>[4x]MGSSHHHHHHSSENLYFQGHIETLPDSFTFYDGTKVQRLSDWPKRAQELKDLYQFYMYGYKPDTSVEDVTYSVNGNTLTITVKVGDKQASFNATVRLPQANSGYQPPYPVIISLGYLAGFNWQTWQFIDYSTNAVNRGYAVISFMPNDVARDDSSYTGAFYTLYPHSNKVENDTGVLMAWAWGASKILDALEKGAIPEIDAKKAIVTGFSRYGKAALVAGAFDERFAVVNPHASGQGGAASFRYSFAGKQYSWGVAGNAEAFSNLQGNTEGHWFNAVFREFKDPRQLPFDQHELIALCAPRTVLITGGYSDWGTNPEGTWVSFVGARKVYEFLGVADRIGFALRDGSHAITEEDVNNLLDFCDWQLRGIQPTKDFSTSRFAIDPAWDTISVPTLYRNAD

The hyperthermophilic bacterium Caldicellulosiruptor kristjansonii encodes an unusual enzyme, CkXyn10C-GE15A, which incorporates two catalytic domains, a xylanase and a glucuronoyl esterase, and five carbohydrate-binding modules (CBMs) from families 9 and 22. C. kristjansonii has been shown to grow on a variety of polysaccharides, including cellulose, xylan, starch, and pectin, with an optimal growth temperature of 78 °C. From the N-terminus, CkXyn10C-GE15A consists of two CBM22 domains (CBM22.1 and CBM22.2), a GH10 endo-xylanase (Xyn10C), three CBM9 domains (CBM9.1, CBM9.2, and CBM9.3), a GE from CE15 (GE15A), a cadherin domain, and two surface layer homology (SLH) domains believed to anchor the protein to the Gram-positive cell wall. Collectively, the results show that all five CBMs have their own distinct binding preferences and appear to complement each other and the catalytic domains in targeting complex cell wall polysaccharides. We have determined the structures of the third CBM9 domain (CBM9.3) and the glucuronoyl esterase (GE15A) by X-ray crystallography.

In addition to determining the structure of CBM9.3, we were also able through renewed efforts to crystallize and determine the structure of the previously biochemically characterized GE15 domain of CkXyn10C-GE15A.15 Residue numbers in this section reflect the numbering as in the PDB file, where Glu22 corresponds to Glu1340 in the full-length protein sequence. We were also able to determine the 3D structure of the GE domain, which represents the first structure of a GE from a hyperthermophilic organism. As expected from previously determined structures of CE15 enzymes, the overall structure is an α/β-hydrolase fold with the active site located in a shallow pocket, and as in other studied bacterial GEs, there are no disulfide bonds. Within the active site, the catalytic serine-histidine-glutamate/aspartate triad is conserved and easily identifiable in CkGE15A and is comprised of Ser210, His348, and Asp311. Compared to previously studied GEs, one of the major differences in CkGE15A is that it lacks two inserts previously found in bacterial enzymes (Reg1 and Reg3) and has a rather different structure of the aromatic-rich Reg2, implicated in the interaction with the lignin portion of the substrate. In the structure of TtCE15A from T. turnerae, rather than a loop, Reg2 is found as a helical protrusion with several aromatic residues that could provide binding sites for complex biomass.22 In CkGE15A, Reg2 is uniquely formed by a β-hairpin, which presents several aromatic residues toward the active site (Phe120, Trp122, Trp125, and Phe127), thus possibly playing a role in substrate recognition and binding moieties such as hydrophobic lignin fragments or a xylan chain. A similarly positioned residue within the loop is not present in CkGE15A due to a sharp turn at Gly115; however, it is possible that Tyr212 could play a similar role, as it is in the same spatial area.> GSARNHTEDNSTEYYDYEEARCACPARHLNNTNGTVLKLLGCHYFCNGTLCTAPDGYPCYNLTAQQVRTLTTYPNTSCAVGVCMKGTCVKNGTMEQCFKTP;> G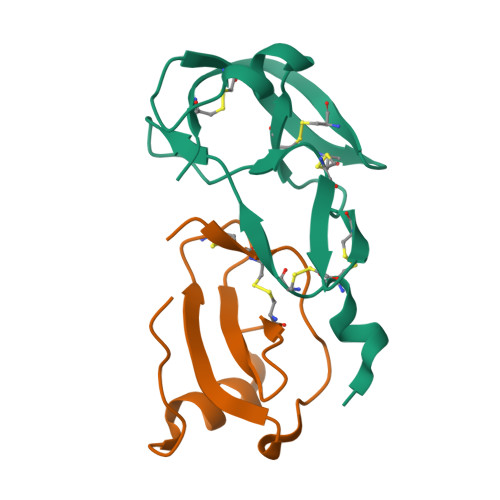PSQPKVPEWVNTPSTCCLKYYEKVLPRRLVVGYRKALNCHLPAIIFVTKRNREVCTNPNDDWVQEYIKDPNLPLLPTRNLSTVKIITAKNGQPQLLNSQ>GSHMPGPVARLAPQAVLTPPSAASLFLVLVAGDSDDDRATVCDVISGIDGPLKAVGFR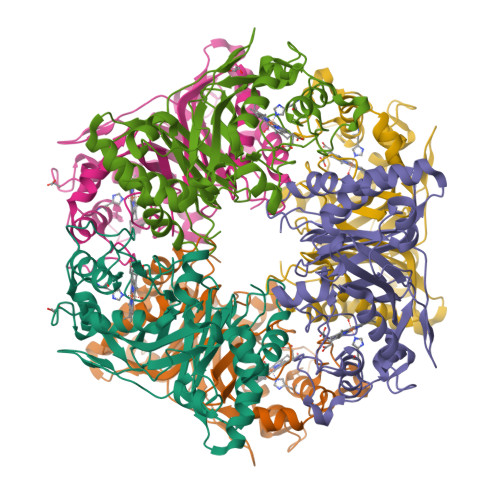ELAGSLSCVVGVGAQFWDRVSASSKPAHLHPFVPLSGPVHSAPSTPGDLLFHIKAARKDLCFELGRQIVSALGSAATVVDEVHGFRYFDSRDLLGFVDGTENPTDDDAADSALIGDEDPDFRGGSYVIVQKYLHDMSAWNTLSTEEQERVIGRTKLENVELDDDAQPSNSHVTLNTIVDDDGVEHDILRDNMAFGSLGEAEYGTYFIGYAKDPAVTELMLRRMFLGEPPGNYDRVLDFSTAATGTLFFVPSRDVLESLGDEPAGAESAPEDPVEPAAAGPYDLSLKIGGLKGVSQ[3x]> GSHMEVTEEDIAEIVSRWTGIPVSKLLEGEREKLLRLEEELHKRVVGQDEAIRAVADAIRRARAGLKDPNRPIGSFLFLGPTGVGKTELAKTLAATLFDTEEAMIRIDMTEYMEKHAVSRLIGAPPGYVGYEEGGQLTEAVRRRPYSVILFDEIEKAHPDVFNILLQILDDGRLTDSHGRTVDFRNTVIILTSNLGSPLILEGLQKGWPYERIRDEVFKVLQQHFRPEFLNRLDEIVVFRPLTKEQIRQIVEIQLSYLRARLAEKRISLELTEAAKDFLAERGYDPVFGARPLRRVIQRELETPLAQKILAGEVKEGDRVQVDVGPAGLVFAVPARVEA

The molecular chaperone ClpB, the bacterial homologue of Hsp104, is a disaggregation machine that provides thermotolerance by resolubilizing and reactivating aggregated proteins in concert with the DnaK (Hsp70) chaperone system. ClpB belongs to the family of AAA+ proteins (ATPases associated with various cellular activities) that comprises a wide range of molecular machines which utilize the energy from ATP hydrolysis to remodel their respective substrates. The AAA+ disaggregation machines Hsp104 and ClpB possess two NBDs per monomer, thus forming double-ring structures with 12 potential ATPase sites in the active hexameric complex. We determined high-resolution X-ray structures in different nucleotide states for one of the motor subunits, namely NBD2, of ClpB and combined the structural analysis with nucleotide-binding kinetics studies.

We therefore crystallized ClpB NBD2 from T. thermophilus under nucleotide-free conditions as well as in the presence of ADP and the nonhydrolysable ATP analogue AMPPCP. Crystallization experiments using 2-propanol as the precipitant yielded well diffracting diamond-shaped crystals for all three states. Structures were determined by molecular replacement to resolutions of 2.8 Å (nucleotide-free), 2.4 Å (ADP) and 1.9 Å (AMPPCP). Most importantly, our structures of the nucleotide-free and AMPPCP-bound states are of significantly higher resolution than those available previously, allowing a more detailed structural analysis. The nucleotide-free structure contained a phosphate ion bound at the same position as the α-­phosphate in the nucleotide-bound structures. This single phosphate ion forms a salt bridge (d = 3.0 Å) with the positively charged side chain of the sensor 2 residue Arg806, which is not observed in the nucleotide-bound states, in which Arg806 is involved in a crystal contact with Glu520 of a neighbouring molecule. Apart from this, the structures of the different nucleotide states are highly similar. Strikingly, in all ClpB NBD2 structures determined to date the side chain of the Walker A lysine Lys601, which is crucial for nucleotide binding and hydrolysis, is present in a completely stretched conformation that prevents the expected interaction with the β/γ-phosphates of the bound nucleotide. Importantly, this inactive picture characterized by a stretched Walker A lysine conformation and the absence of Mg2+ from the catalytic site is not only observed in our structures but also in all other ClpB NBD2 structures published to date, independent of the nucleotide state.> GSGSAMIEARQVSELSTRIISSVQMLSNAQNEQERKEAGRVLFEQLESLLTHIKELGGESFDSKLLDALESNVQNVINNLAELGVTVERKLWLAKEIDTRVEEMRLLSEELEQLTRTQVQNTSTIAVANVTHIYDLLEANKKDQVYQALDALVEVDLDLTERLHELHLLAFKMLNQIEEARTLTNVDRIQQIQTAFENNLKIMKRRVLAVEDPTRSKQMSQLLTELGKRQVVFTILLQQYENNEQSQQLMQKTLELFSELNSTVNKLVDDSNKTTTK;> GSGSDEKICAIYPHLKDSYWLSVNYGMVSEAEKQGVNLRVLEAGGYPNKSRQEQQLALCTQWGANAIILGTVDPHAYEHNLKS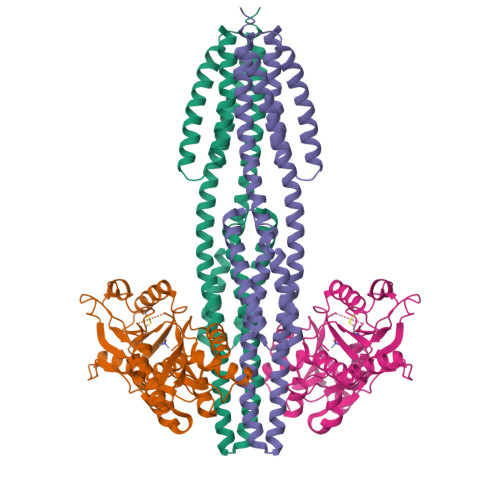WVGNTPVFATVNQLDLDEEQSTLLKGEVGVDWYWMGYEAGKYLAERHPKGSGKTNIALLLGPRTRGGTKPVTTGFYEAIKNSDIHIVDSFWADNDKELQRNLVQRVIDMGNIDYIVGSAVAIEAAISELRSADKTHDIGLVSVYLSHGVYRGLLRNKVLFAPTDKMVQQGRLSVMQAAHYLRHQPYEKQASPIIKPLTPKTLHDDTIEESLSPSEYRPTFS> EEDLTEVKKDALENLRVYLCEKIIAERHFDHLRAKKILSREDTEEISCR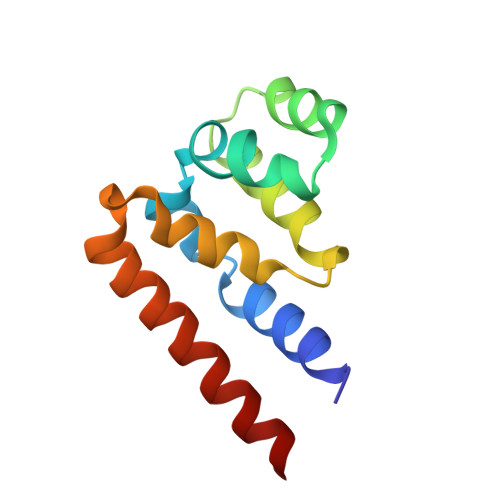TSSRKRAGKLLDYLQENPKGLDTLVESIRREKTQNFLIQKITDEVLKLRNIKLEHLK7-methyl-3,4-dihydro-2~{H}-pyrido[1,2-a]pyrimidin-3-ol | C9 H12 N2 O | 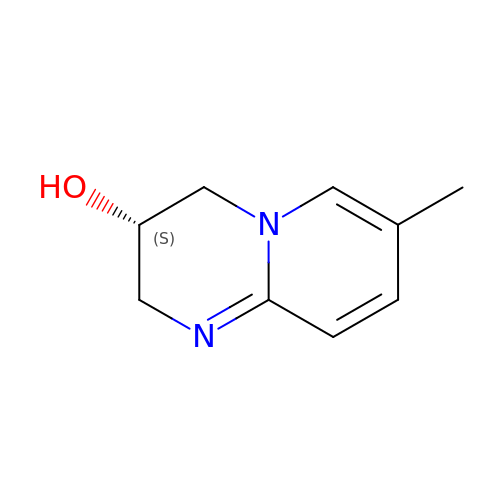ZXHXLZFWEYQXTL-QMMMGPOBSA-N>[3x]MKGFNIYTDESTLVSIGDDAGVYEHNGIIWVYTVDIITPVVNDPYLWGAISTANALSDVYAMGGIPVNALAISCFNNCELDIEIFREVIRGALDKLREAKTVLLGGHTIDDKEPKFGLSVAGICPEGKYITQSGAQVGQLLILTKPIGTGILIKGLKEGILKEEDINEAIENMLALNDKARNLMLSLDATACTDVTGFGLLGHAWNICK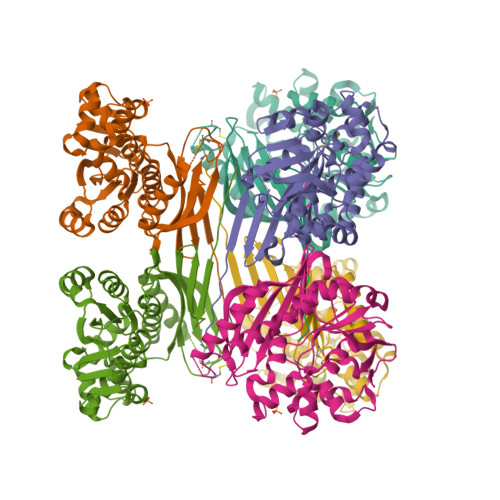NSNIGARIFFEKVPYYQLSENLVKKKIYPKGAIENLNFVKNYLKSNLDNWKLILLSDPVTSGGLLFTINKEKLEKIDETAKELEVNYWIIGETIAENVLEVL>[2x]MLEGLVAGLLNRFLGMYVKNFDPKQLKWEVWNGKVRLDNLELQREALDQLKLPINVIKGHLGHLVLHIPWKTLASEQVKINIEDVFLLASPKEEAEYDEDEEARRRHRLKMEKLDSAELLKERSQEGLSEEEQKRTQTFAQALVTKIVDNLQITIRNIHIRYEDAISAPGHPFALGITLEEFSAVSTDSDWTPAFITS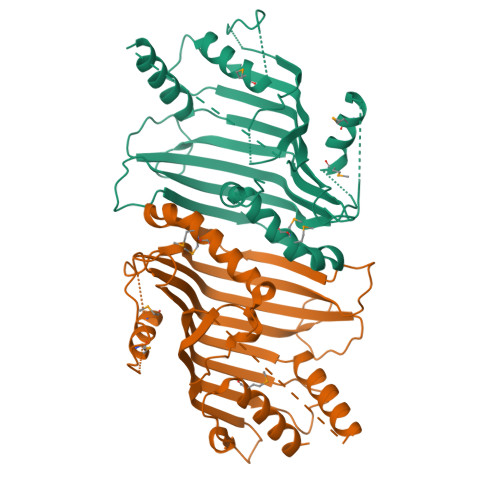IQSAHKLATLESLAIYWDTDAKLIGPGREHHEHDEMLKFFREMIAKGEADLSSEHQFILKPVSGQAKIEIDKTGSHTVPRYKANLLFDEIGVVLDDQQYRDALMMVDLFHYFIRHQEYKKFQPKGVTPKEDGHHHHHH> MAGDD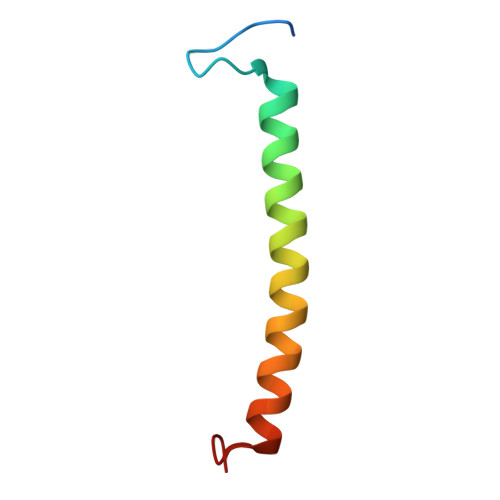TKVYPTGLTEAQALEINDGLKWGTRIYFGIAVAAHILAFILTPWLK>[30x]MADALGMIEVRGFVGMVEAADAMVKAAKVELIGYEKTGGGYVTAVVRGDVAAVKAATEAGQRAAERVG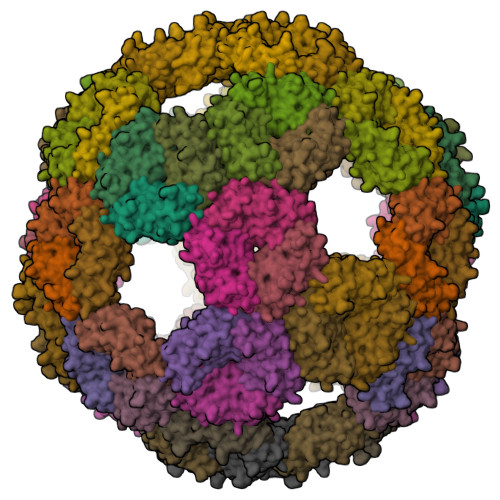EVVAVHVIPRPHVNVDAALPLGRTPGMDKSALDAPVVADAWEEDTESADALGMIEVRGFVGMVEAADAMVKAAKVELIGYEKTGGGYVTAVVRGDVAAVKAATEAGQRAAERVGEVVAVHVIPRPHVNVDAALPLGRTPGMDKSA> SDRVAQLTIGNSTITTQEAANIIVGYGEWPSYCSDDDATAVDKPTRPDVSVNRFYTLDTKLWEKSSKGWYWKFPDVLTETGVFGQNAQFHYLYRS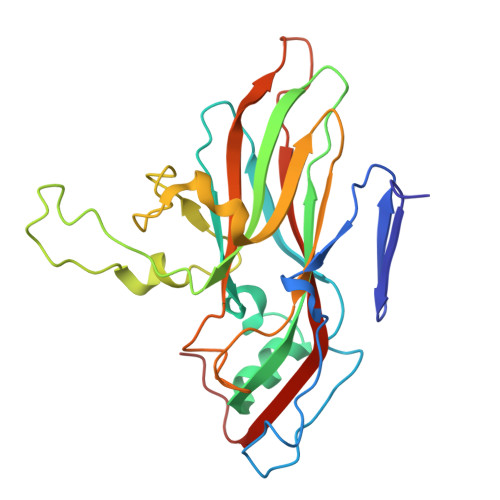GFCIHVQCNASKFHQGALLVAILPEYVIGTVAGGTGTEDSHPPYKQTQPGADGFELQHPYVLDAGIPISQLTVCHHQRINLRTNNCATIIVPYMNTLPFDSALNHCNFGLLVVPISPLDFDQGATPVIPITITLAPMCSEFAGLRQAVTQ>MKAYTKYLTFNTKKRRELIRITDEVKKAVEESEVKEGLCLVSSMHLTSSVIIQDDEEGLHEDIWEWLEKLAPYRPDYKHHRTGEDNGD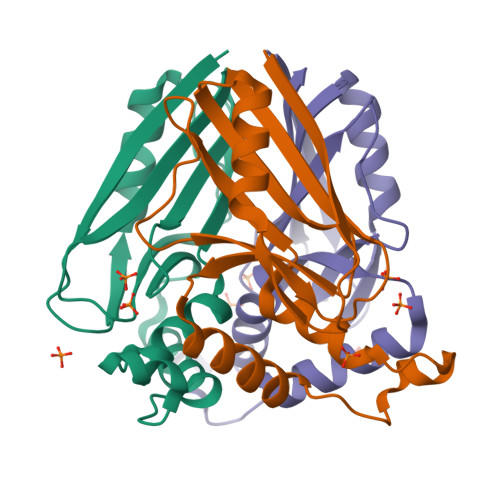AHLKNLLTHLQVVLPITNGKLDLGPWQEIFYAEFDGQRPKRVVIKIIGE[2x]The large (L) protein of LASV is a multi-domain molecular machine that binds the conserved 3′ and 5′ ends (the ‘promoter’) of each of the two viral RNA (vRNA) genome segments (denoted L and S) and plays a central role in the viral life cycle, which is entirely cytoplasmic. The L protein contains an RNA-dependent RNA polymerase (RdRp) activity and catalyses both viral transcription and genome replication. Transcription is initiated using a capped primer derived from host mRNA by a yet to be elucidated ‘cap-snatching’ mechanism involving the intrinsic endonuclease (EN) of the L protein and possibly its cap-binding domain (CBD).

From grids of the apo-state, two different 3D classes were separated. In the second class, denoted APO-RIBBON, at 3.73 Å resolution, the EN is not resolved, but residues 822–1110 of the L protein form an extended structure including an α-bundle (α-ribbon, 843–884, with a third helix 907–925 packing against it) that is not visible in the APO-ENDO structure. Masked refinement of the common regions of the two apo-structures yielded a map of the APO-CORE with an improved resolution of 3.14 Å that allowed a more accurate model to be built.

> MEDDMACVKDLVSKYLADNERLSRQKLAFLVQTEPRMLLMEGLKLLSLCIEIDSCNANGCEHNSEDKSVERILHDHGILTPSLCFVVPDGYKLTGNVLILLECFVRSSPANFEQKYIEDFKKLEQLKEDLKSVDINLIPLIDGRTSFYNEQIPDWVNDKLRDTLFSLLRYAQESNSLFEESEYSRLCESLSMTSGRLSGVESLNVLLDNRSSHYEEIIASCHQGINNKLTAHEVKLQIEEEYQVFRNRLRKGEITGQFLKVDKSRLLNDFNNLYVDEVTATKDNIEHLIYQFKRASPILRFLYANIGEGNGEERHHTIKECQMQYWRSFLNKVKSLRILNTRRKLLLIFDALILLASIHDQTRHKCSKGWLGSCFISVNDRLVSLESTKRDLEKWVGRRQQSERSNTIQPPDKNQILISMFQKTILKATAALKDVGISVEHYKINMEVICPDSYDLILNFDVSGVVPTISYQRTEDEKFPFIMGGVELLESTDLERLSSLSLALVNSMKTSSTVKLRQNEFGPARYQVVRCKEAYCQEFLLSGAEFQLIYQKTGECSKCYAINDNRVGEICSFYADPKRYFPAIFSAEVLQTTVSTMISWVKDCSELEEQLCNINSLTKMILVLILAHPSKRSQKLLQNLRYFIMAYVSDYHHKDLIDKLREELITDVEFLLYRLVRALVNLILSEDVKSMMTNRFKFILNISYMCHFITKETPDRLTDQIKCFEKFLEPKLEFGHVSINPADVATEEELDDMVYNAKKFLSKEGCTSIKGPDYKKPGVSKRFLSLLTSSFNNGSLFKESEVKREIKDPLVTSGCATALDLASNKSVVVNKYTDGSRVLNYDFNKLTALAVSQLTEVFSRKGKHLLNKQDYDYKVQQAMSNLVLGPRQNKVGADEADLDEILLDGGASVYFDQLKETVERIIDQYREPVKPGSNPNGGDQPSVNDLDEVVPNKFYIRLIKGELSNHMVEDFDYDVLPGNFYEEFCDAVYKNNKLKERYFYCGQMSQCPIGELTKAVATRTYFDQEYFQCFKSILLIMNANTLMGRYTHYKSRNLNFKFDMGRLSDDVRISERESNSEALSKALSLTNCTTAMLKNLCFYSQESPQSYSSTGPDTGRLKFSLSYKEQVGGNRELYIGDLRTKMFTRLIEDYFEALSLQLSGSCLNNEREFENAILSMKLNVSLAHVSYSMDHSKWGPMMCPFLFLATLQNLIFLSKDLQADIKGRDYLSTLLTWHMHKMVEIPFNVVSAMMKSFIKAQLGLKKKTTQSITEDFFYSNFQIGVVPSHVSSILDMGQGILHNTSDFYALISERFINYAISCICGGTIDAYTSSDDQISLFDQVLTELMQRDPEEFKTLIEFHYYMSDQLNKFVSPKSVIGRFVAEFKSRFYVWGDEVPLLTKFVAAALHNIKCKEPHQLAETIDTIIDQSVANGVPVHLCNLIQKRTLSLLQYARYPIDPFLLNCETDVRDWVDGNRSYRIMRQIERLIPDACGRIRSMLRKLYNKLKTGQLHEEFTTNYLSSEHLSSLSNLCELLGVEPPSESDLEFSWLNLAAHHPLRMVLRQKIIYSGAVNLDDEKVPTIVKTIQNKLSSTFTRGAQKLLSEAINKSAFQSSIASGFVGLCRTLGSKCVRGPNKESLYIKSIQSLISDIQGIEPLIDSHGVQYWRVPLNIRDGNEGVISYFRPLLWDYMCISLSTAIELGAWVLGEPKKVRVLEFFKHNPCDYFPLKPAASKLLEDRVGLNHIIHSLRRLYPSVFEKHILPFMSDLASTKMKWSPRIKFLDLCVALDVNCEALSLVSHIVKWKREEHYIVLSSELRLSHTRTHEPMVEERVVSTSDAVDNFMRQIYFESYVRSFVATTRTLGSFTWFPHKTSVPEGEGLQRLGPFSSFVEKAIHKGIERPMFKHDLMMGYAWIDFDIEPARFNHNQLIASGLVGPRFDSLEDFFDAVESLPPGSAKLSQTVRFRIKSQDASFKESFAIHLDYTGSINQQTKYLVHEVSAMYSGAVSPCVLSDCWRLVLSGPTFKGKSAWYVDTEIVNEFLTDTNQLGHVTPVEIVVDMEKLQFTEYDFVLVGPCVEPVPLVVHRGGLWECDKKLASFTPVVQDQDLEMFVKEVGDSSLDLLIGALSAMILDRLKLRMQWSEVDIVSMLKAAMPSNSVKVLNAVLEAVDDWVDFKGYALCYSKSRKKVMVHSSGGKLRLKGRTCEELVKEDEGIEDIE>MSSAIKEVQGAPVKWVTNWTPEAIRGLVDQEKGLLDPRIYADQSLYELELERVFGRSWLLLGHESHVPETGDFLATYMGEDPVVMVRQKDKSIKVFL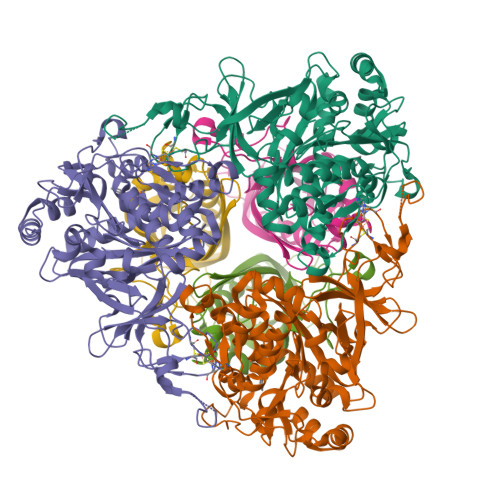NQCRHRGMRICRSDAGNAKAFTCSYHGWAYDIAGKLVNVPFEKEAFCDKKEGDCGFDKAEWGPLQARVATYKGLVFANWDVQAPDLETYLGDARPYMDVMLDRTPAGTVAIGGMQKWVIPCNWKFAAEQFCSDMYHAGTTTHLSGILAGIPPEMDLSQAQIPTKGNQFRAAWGGHGSGWYVDEPGSLLAVMGPKVTQYWTEGPAAELAEQRLGHTGMPVRRMVGQHMTIFPTCSFLPTFNNIRIWHPRGPNEIEVWAFTLVDADAPAEIKEEYRRHNIRNFSAGGVFEQDDGENWVEIQKGLRGYKAKSQPLNAQMGLGRSQTGHPDFPGNVGYVYAEEAARGMYHHWMRMMSEPSWATLKP[12x];>MTNPSPHFFKTFEWPSKAAGLELQNEIEQFYYREAQLLDHRAYEAWFALLDKDIHYFMPLRTNRMIREGELEYSGDQDLAHFDETHETMYGRIRKVTSDVGWAENPPSRTRHLVSNVIVKETATPDTFEVNSAFILYRNRLERQVDIFAGERRDVLRRADNNLGFSIAKRTILLDASTLLSNNLSMFF[12x]> MRYPESLLKLTRALSRLPGIGPKTAQRLALHLAFHKEEAEALAEALEGIKRVRACRECGNLAEGELCPICQDEDRDRSLLAVVESVADLYALERSGEFRGLYHVLGGALNPLEGIGPKELNLEGLFRRLEGVEEVVLATS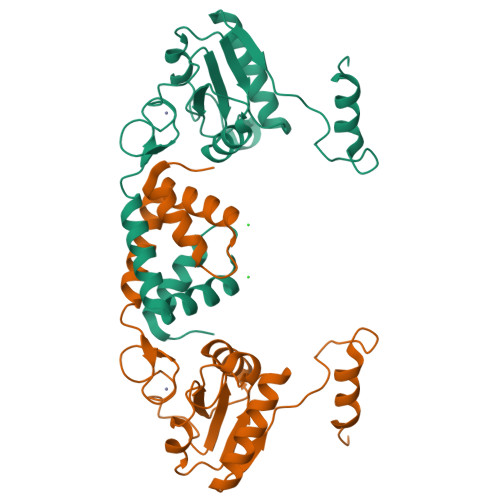MTVEGEATALYLAEELKKRGVRVTRPAYGLPVGGSLEYADEVTLGRALEGRRPV2-[4-(1~{H}-pyrazol-3-yl)phenoxy]pyrimidine | C13 H10 N4 O | 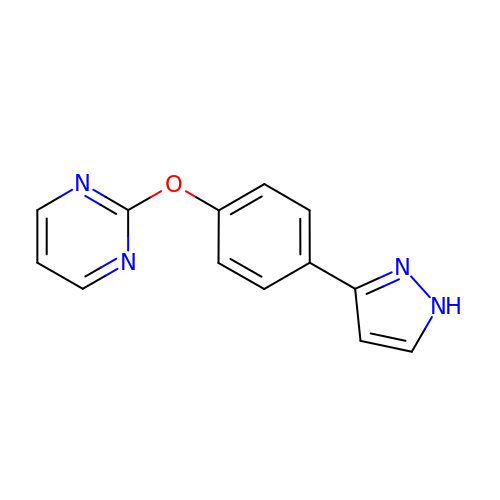DUEUESIXAVJTRZ-UHFFFAOYSA-N N,N'-(octane-1,8-diyl)bis(2,2-dichloroacetamide) 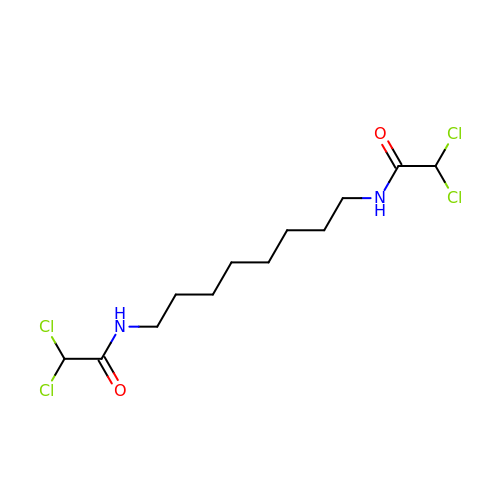| C12 H20 Cl4 N2 O2 | FAOMZVDZARKPFJ-UHFFFAOYSA-N>MGSSHHHHHHSSGENLYFQGEAVVISGRKLAQQIKQEVRQEVEEWVASGNKRPHLSVILVGENPASHSYVLNKTRAAAVVGINSETIMKPASISE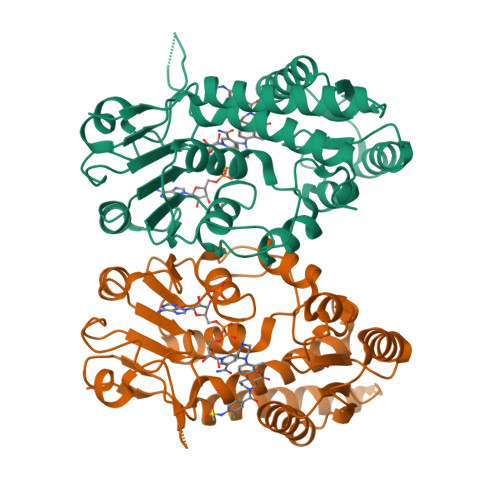EELLNLINKLNNDDNVDGLLVQLPLPEHIDERRICNAVSPDKDVDGFHVINVGRMCLDQYSMLPATPWGVWEIIKRTGIPTLGKNVVVAGRSKNVGMPIAMLLHTDGAHERPGGDATVTISHRYTPKEQLKKHTILADIVISAAGIPNLITADMIKEGAAVIDVGINRVHDPVTAKPKLVGDVDFEGVRQKAGYITPVPGGVGPMTVAMLMKNTIIAAKKVLRLEERE[2x]> SSLSPYLRYLPSDVSGGEWDKPDVGDVLC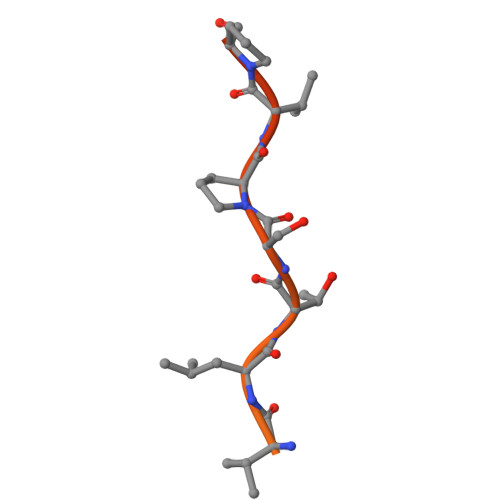FQAKEPQRRRVLTSPVPDELLIK> HMGSDGTWELSVHVTDLNRDVTLRVTGEVHIGGVMLKLVEKLDVKKDWSDHALWWEKKRTWLLKTHWTLDKCGIQADAKLQFT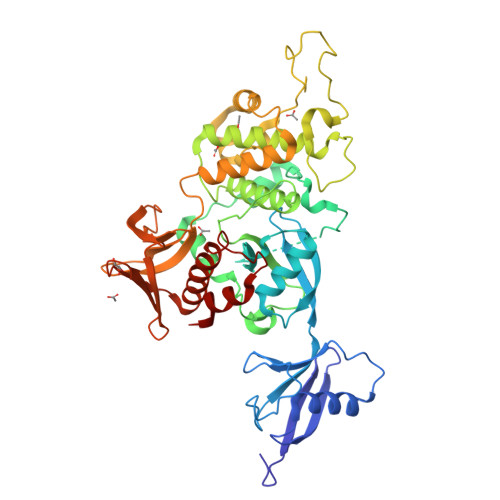PQHKLLRLQLPNMKYVKVKVNFSDRVFKAVSDICKTFNIRHPEELSLLKKPRDPTKKKKKKLDDQSEDEALELEPGILAVSQPVTSPEILAKMFKPQALLDKAKTNQGWLDSSRSLMEQDVKENEALLLRFKYYSFFDLNPKYDAIRINQLYEQAKWALLLEEIECTEEEMMMFAALQYHINKLSIMTSENHLNNSDKEVDEVDAALSDLEITLEGGKTSTILTTDVNPECLVSPRYLKKYKSKQITARILEAHQNVAQMSLIEAKMRFIQAWQSLPEFGITHFIARFQGGKREELIGIAYNRLIRMDASTGDAIKTWRFSNMKQWNVNWEIKMVTVEFADEVRLSFICTEVDCKVVHEFIGGYIFLSTRAKDQNESLDEEMFYKLTSGWV>GSHMDLGAPQNPNAKAAGSRKIHFNWLPPSGKPMGYRVKYWIQGDSESEAHLLDSKVPSVELTNLYPYCDYEMKVCAYGAQGEGPYSSLVSCRTHQEVPSEPGRLAFNVVSSTVTQLSWAEPAETNG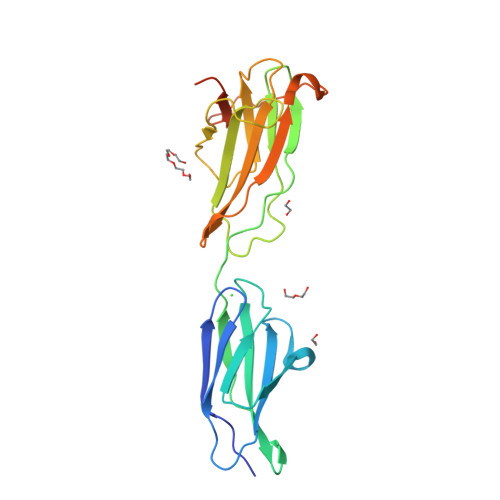EITAYEVCYGLVNDDNRPIGPMKKVLVDNPKNRMLLIENLRESQPYRYTVKARNGAGWGPEREAIINLATQPKRPMSIPIIPDIPIVDAQSGEDYDSFLMYSDDVLR[2x]> LMLLPNILLTGTPGVGKTTLGKELASKSGLKYINVGDLAREEQLYDGYDEEYDCPILDEDRVVDELDNQMREGGVIVDYHGCDFFPERWFHIVFVLRTDTNVLYERLETRGY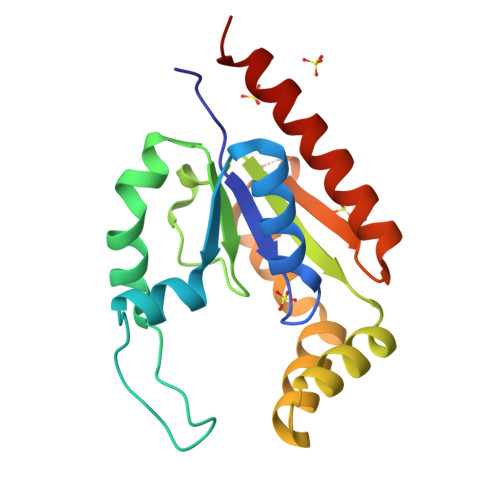NEKKLTDNIQCEIFQVLYEEATASYKEEIVHQLPSNKPEELENNVDQILKWIEQWIKDHNS> TGFNLSIDTVEGNPGSSVVVPVKLSGISKNGISTADFTVTYDATKLEYISGDAGSIVTNPGVNFGI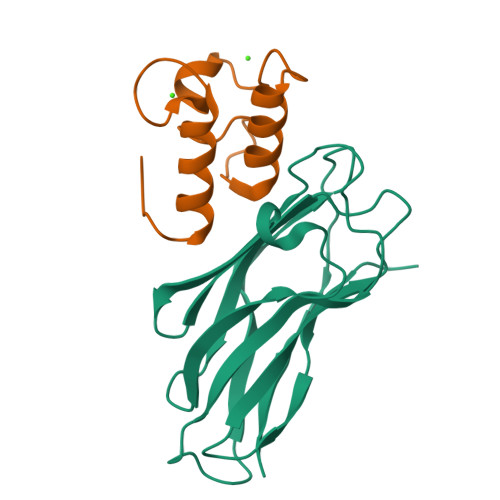NKESDGKLKVLFLDYTMSTGYISTDGVFANLNFNIKSSAAIGSKAEVSISGTPTFGDSTLTPVVAKVTNGAVNLE;> KPGDVDGNGSINSIDFALMRNYLLGNLKDFPAEDDIKAGDLNGDKSININDFAIMRMYLLGMITKF>MASMTGGQQMGRGSMAADILVVDDEVDIRDLVAGILSDEGHETRTAFDADSA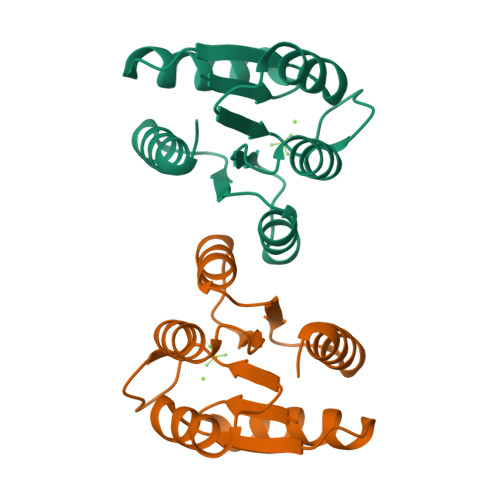LAAINDRAPRLVFLDIWLQGSRLDGLALLDEIKKQHPELPVVMISGHGNIETAVSAIRRGAYDFIEKPFKADRLILVAERALETSKLKLEHHHHHH[2x]>[2x]GMMQKPITEIIIVGGGTAGWITAGLLAAEHNVDKGVLAHSPKLNITLIESPDVATIGVGEGTWPSMRSTLSKIGIDENDFIRQCDASFKQGSRFINWCKDPQSNVADSYLHPFSLPHGHQELDLCPYWLPHAEQVSFAEAVCSQQVLTQLGLAPKSIVTAQYHFQNNYGYHLNAAKFSQLLTEHCTQKLGVTHIRDHVSQIINNQHGDIEKLITKQNGEISGQLFIDCTGAKSLLLGEHLQVPFLSQKSVLFNDRALAIQVPYSDANSPI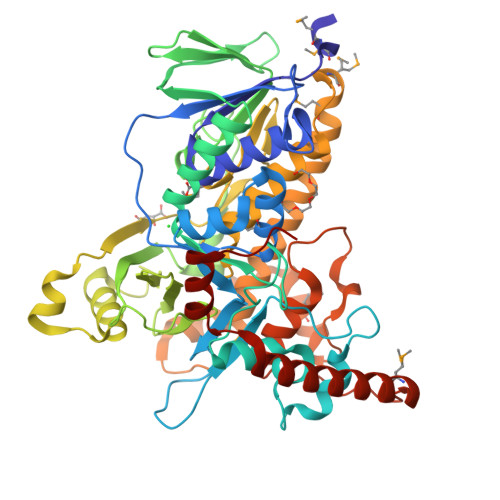ASCTHSTAQPNGWIWDIGLPTRKGVGYVYSSSHTNDIDAQKTLFNYLGVDGAAADKLEPRQLAINPGYRAKCWQNNCIAIGMAAGFIEPLEASALALIEWTASTLAQQLPPNRMVMDTISARVNERYQQHWQQIIDFLKLHYVISQRQEDRYWRDHRESNSIPDSLQAMLELWRYQTPSQQDISYKEALFPAASFQYVLYGMSFNTQLPTHVKPSMQQLAQRLFNDNQQRTQALSKNLPTNRELLDKVAQYGFPKL> M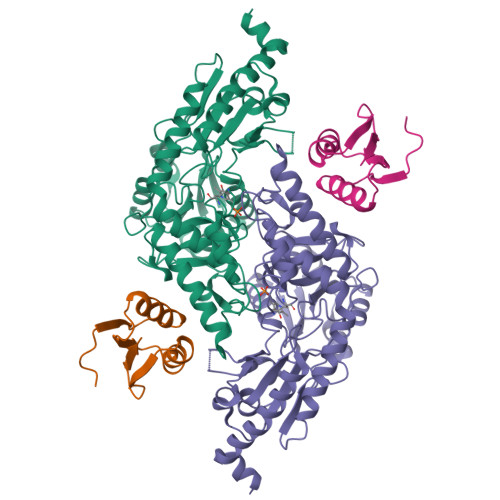GSSHHHHHHGSMYGVYRAMKLPIYLDYSATTPVDPRVAEKMMQFMTMDGTFGNPASRSHRFGWQAEEAVDIARNQIADLVGADPREIVFTSGATESDNLAIKGAANFYQKKGKHIITSKTEHKAVLDTCRQLEREGFEVTYLAPQRNGIIDLKELEAAMRDDTILVSIMHVNNEIGVVQDIAAIGEMCRARGIIYHVDATQSVGKLPIDLSQLKVDLMSFSGHKIYGPKGIGALYVRRKPRVRIEAQMHGGGHERGMRSGTLPVHQIVGMGEAYRIAKEEMATEMERLRGLRNRLWNGIKDIEEVYLNGDLEHGAPNILNVSFNYVEGESLIMALKDLAVSSGSACTSASLEPSYVLRALGLNDELAHSSIRFSLGRFTTEEEIDYTIELVRKSIGRLRDLSPLWEMYKQGVDLNSIEWAHH;> GSTDLFSSPDHTLDALGLRCPEPVMMVRKTVRNMQPGETLLIIADDPATTRDIPGFCTFMEHELVAKETDGLPYRYLIRKGG>[4x]MFPARLSLAVLFSVSPALAYFSGLGLGSERSIFRRDLNSTGDESNSTQWPAPLANGGKSWASAFKKAKATVTEMTVEELANITSGVIGLCSGVTGAV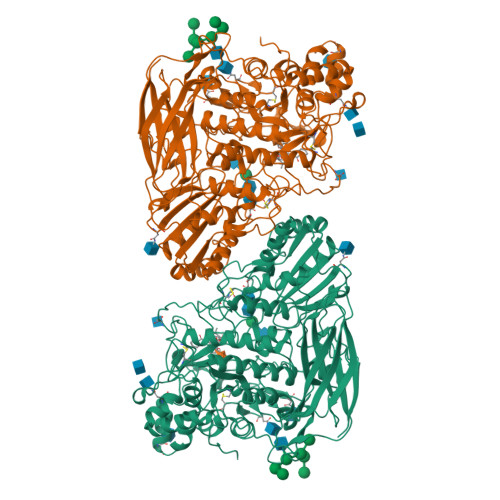TRLGIPEFCLQDGPIGPRGVHGSSQFPAGLTVAATWDRTLMYARARGMGQEFHDQGVHLALAPVTGGPLGRTPLNGRGWEGTFADPYACGEASYLSVKGLTDAGVATVSKHWIAYEQETSRNLYIDIDGVSQADIQLPISSNVDDLTMHELYMWSFAEAVRAGTNHIMCSYNRINNTHSCSNAKGLNQLLKTELNFQGGVVSDWGGQWDSVPAAENGLDVAMPGKGFLGALGDFWGATLVELINNGTVSEDLVRDKAVRILTGYYYLGQDTNPPPPFVYNTIGAPTLNATSGYRNVRKPGTAELIKEIGSASVTLLKNTGSLPLKHPQRIAVLGNDATYNVLGPNACGLANSACDIDNLNGTLTTGGGSGSALSPYTITPLEALQKRAIEDNAEIAAVVANSNTTTGAEDAIAALLPDADVTFVFLNRYSEEGADAPDFSLGGDGDNLMDLAVTYSSNVVVVIHTTGVVDIEKWADNPNVTAILVAYLPGQEAGNSLVPVLYGDVAPSGKLPWTWGKSIDDYVPNGVVYTDAYSPQSNFTEGVFIDYRWFDKMGITPRYEFGFGLSYTTFTYSNLIVDHGRWAKDYSSVMETAEPFAEWDGTNSLYDVIFTVFATITNTGNLTGSEVAQLYISIPGDNQPVRQLRGFDKIKDLPVGDSAVVTFPIRRKDVSSWSVVDQLWYVPNGDFLISVGGSSRDLPLNTTWTP>[3x]TINVTGDGNVFKPSAETSSTAVPSLSLSPGMLNPGGVPWIAIGDETSVTSPGALRRMTSKDIDEPLVVVTEHAIANFTKAEMALEFNREFLDKLRVLSVSPKYSDLLTYVDCYVGVSARQALNNFQKQVPVITPTRQTMYVDSIQAALKALEKWEIDLRVAQTLLPTNVPIGEVSCPMQSVVKLLDDQLPDDSLIRRYPKEAAVALAKRNGGIQWMDVSEGTVMNEAVNAVAASALAPSASAPPLEEKSKLTEQAMDLVTAAEPEIIASLVPVPAPVFAIPPKPADYNVRTLKIDEATWLRMIPKTMGTLFQIQVTDNTGTNWHFNLRGGTRVVNLDQIAPMRFVLDLGGKSYKETSWDPNGKKVGFIVFQSKIPFELWTAASQIGQATVVNYVQLYAEDSSFTAQSIIATTSLAYNYEPEQLNKTDPEMNYYLLATFIDSAAITPTNMTQPDVWDALLTMSPLSAGEVTVKGAVVSEVVPAELIGSYTPESLNASLPNDAARCMIDRASKIAEAIKIDDDAGPDEYSPNSVPIQGQLAISQLETGYGVRIFNPKGILSKIASRAMQAFIGDPSTIITQAAPVLSDKNNWIALAQGVKTSLRTKSLSAGVKTAVSKLSSSESIQNWTQGFLDKVSTHFPAP;>MEVCLPNGHQIVDLINNAFEGRVSIYSAQEGWDKTISAQPDMMVCGGAVVCMHCLGVVGSLQRKLKHLPHHRCNQQIRHQDYVDVQFADRVTAHWKRGMLSFVCQMHAMMNDVSPEDLDRVRTEGGSLVELNWLQVDPNSMFRSIHSSWTDPLQVVDDLDTKLDQYWTALNLMIDSSDLVPNFMMRDPSHAFNGVRLEGDARQTQFSRTFDSRSSLEWGVMVYDYSELEHDPSKGRAYRKELVTPARDFGHFGLSHYSRATTPILGKMPAVFSGMLTGNCKMYPFIKGTAKLKTVRKLVDSVNHAWGVEKIRYALGPGGMTGWYNRTMQQAPIVLTPAALTMFSDTTKFGDLDYPVMIGDPMILG[3x]

The particles harbour 10-separate genome segments and comprise two principle protein layers, the innermost composed of 120 copies of protein λ1 clamped together by 150 copies of σ2 (viral polymerases, λ3, are attached inside adjacent to the icosahedral fivefold axes). The outer layer consists of 600 copies each of μ1 and σ3. The array of μ1 and σ3 is interrupted at the fivefold axes by pentameric λ2 turrets which enzymatically cap the mRNA transcripts produced by the polymerase on egress from the particle. Here we demonstrate that vitrification of infected cells followed by cryo-focussed ion beam (cryo-FIB) milling and cryo-electron tomography (cryo-ET) allows high resolution reconstruction of assembly intermediates of a mammalian reovirus, allowing atomic models to be constructed which throw light on some of these fundamental questions.

In addition virion-like particles of two types, ‘empty’ and ‘full’, were observed. The two virion-like particles are extremely similar, with the exception that the density level is much higher in the interior of the full particles. For stars, analysis focused on the fivefold regions using emClarity16 yielded a reconstruction at 6.6 Å. For the empty virion-like particles, reconstructions focused on the fivefold regions and pseudo sixfold regions yielded reconstructions at 6.5 and 5.6 Å respectively. We believe that cryo-ET of suitably prepared infected cells will be a general vehicle for understanding virus replication-cycles in atomic and molecular detail, with our study already providing a reconstruction at 5.6 Å resolution from only 65 icosahedral particles. If there is indeed some similarity in the assembly process, with collapsed particles being transformed into an expanded state by the recruitment of the RNA genome then the empty virion-like particles we observe would be dead-end products that have failed to package the genome. Indeed the proportion of empty virion-like particles observed is consistent with the known ~50% failure rate in packaging observed in strains which do not organize their virus factories in association with cellular microtubules.> ASMTGGQQMGRGSSLTACPEESPLLVGPMLIEFNIPVDLKLVEQQNPKVKLGGRYTPMDCISPHKVAIIIPFRNRQEHLKYWLYYLHPILQRQQLDYGIYVINQAGESMFNRAKLLNVGFKEALKDYDYNCFVFSDVDL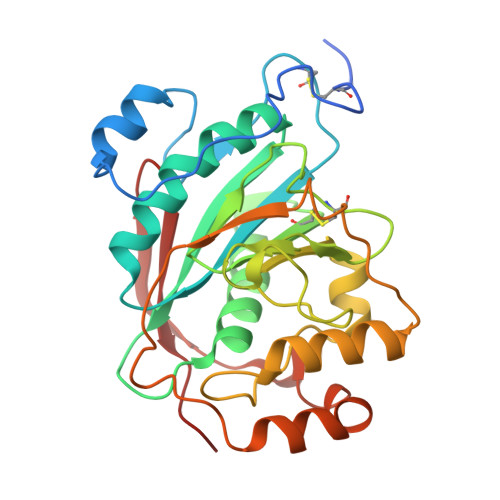IPMNDHNTYRCFSQPRHISVAMDKFGFSLPYVQYFGGVSALSKQQFLSINGFPNNYWGWGGEDDDIYNRLAFRGMSVSRPNAVIGKCRMIRHSRDKKNEPNPQRFDRIAHTKETMLSDGLNSLTYMVLEVQRYPLYTKITVDIGTPS> KETAAAKFERQHMDSSTSAASSSNYCNQMMKSRNLTKDRCKPVNTFVHESLADVQAVCSQKNVACKNGQTN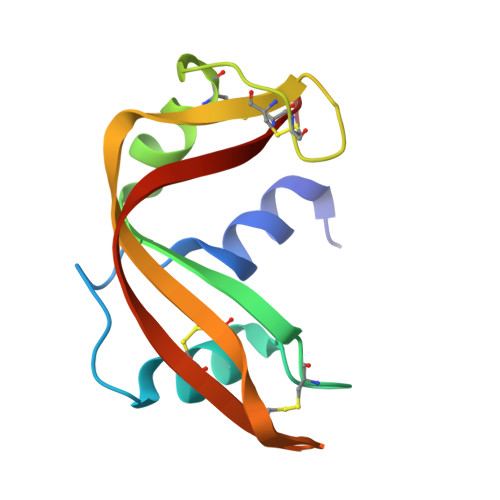CYQSYSTMSITDCRETGSSKYPNCAYKTTQANKHIIVACEGN>[2x]TGQLQEQKKGLLIAVSVSVDKIISHFGAA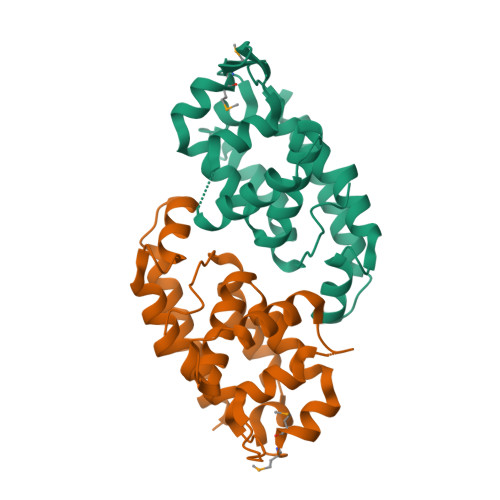RNLVQKAQLGDSRLSPDVGHLVLTTLCPALHALVADGLKPFRKDLITGQRRSSPWSVVEASVKPGSSTRSLGTLYSQVSRLAPLSSSRSRFHAFILGLLNTKQLELWFSSLQEDAGLLSLMYMPTGFFSLARGGCPSLSTELLLLLQPLSVLTFHLDLLFELEHHHHHH> MKKIILGLSVLCLLMACGSSEQPAVIKVSEETLMYEVRATPSPADGTYVKVNPPRFMWPDKFPHLGPVLDGVPGQVDEKPKVVYRIRISQDKNFRKDVLTGERAWAFFNPFQCLAQGKWYWQHAYVTPEGTEEWSPVYQFYIDKDTPEFNPPTLEKVLARYPSHHPRVLLDADDWENIIAKNNNNPEARTYMDKASQCISRPLKHLQEEIDTTNVVTLTNI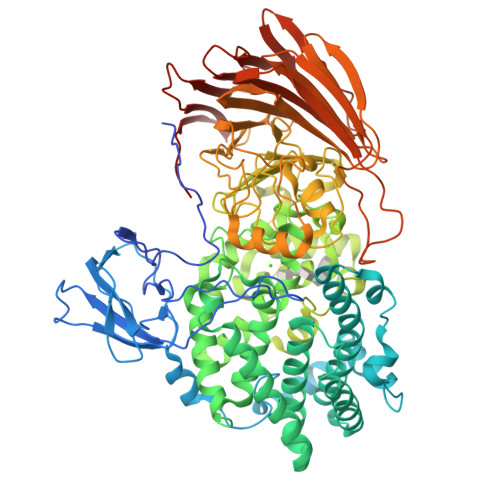VQRESALIRESRKIVDREEANVEALVRAYLLTKDEKYYREGINRLSEILSWQKSKYFAGDFNLSTLLSMSTSAYDGFYNLLSPEEKQLLLDNIRKIGDKFYNEYVNHLENRIADNHVWQMTFRILTMAAFATVGEIPEASVWTDYCYNEWISRLPGLHKDGGWHNGDAAFHVNIRTLIEVPVFFSRISGFNFFADPWYNNNALYVIYQQPPFSKSGGHGNSHEGQRSPNGGRIGYADALARECNNPWAAAYVHEIMQEDPDILSKAFEAKPADLTWYRCTTPKERPAYSKHLSELPESKVFKQTGTALMNTDIGHHANNAMLSFRSSPYGSTSAALANQNAFNTFFGGKAIFYSSGHRTGFTDDHCMYAYRNTRAHNSILVNGMGQKIGTEGYGWIPRYYEGEEISYVVGDASNAYGKVVSPLWLERGRLSGTQFTPEKGWDENKLEFFRRHVVQLGRSGLFVVYDELAGKEPVEWNYLLHTVELPMEVVKEEGGLRILGKNKADGISIAHLYSSQEMTYAQTDTFFVAALDWKKRLGKALPNHYHFTATTAPCNKVFFLNIIDVHGNNRADAVINHQGNHITVEGWVIECNLDSEGKAFLHIENKQNGASLDFNYNSNKGATTIVDQVDGKRIEKRLVDSLPEPEILEHHHHHH Mpf2Ba1 is a 53.2 kDa protein isolated from Pseudomonas monteilii through a multi-step purification process informed by artificial diet bioactivity screening against WCR larvae. The protein is comprised of two domains—an N-terminal MACPF domain and a C-terminal β-prism domain. Pore-forming proteins (PFPs) are a major class of soluble proteins that oligomerize into rings and undergo large irreversible conformational changes to become transmembrane assemblies and breach the membrane of target cells. We have identified and characterized the non-Bt insecticidal protein Mpf2Ba1, providing mechanistic details for how it effectively kills the devastating maize pest WCR by forming pores in midgut membranes targeting a different binding site than the insecticidal proteins currently deployed in commercial transgenic maize hybrids.

A major finding that facilitated Mpf2Ba1 structural characterization is that gut fluid extracted from WCR larvae is necessary and sufficient to induce oligomerization in vitro in the absence of brush-border membrane vesicles (BBMVs) prepared from isolated gut tissue. Upon incubation in gut fluid, an N-terminal cleavage after Lys25, as determined through Edman degradation sequencing, and subsequent oligomerization step are triggered by interaction of monomers with yet unidentified midgut component(s). After gut fluid-induced oligomerization, Mpf2Ba1 monomers formed higher-order complexes that were isolated via size exclusion chromatography and imaged by cryo-EM. The 3D reconstruction of ring-shaped oligomers at 3.1 Å resolution revealed an intermediate state of Mpf2Ba1: a 22-mer pre-pore that is 80 Å in height, 260 Å in diameter, and encircles a 120 Å-wide lumen. By fitting and refining the X-ray structure of Mpf2Ba1 into the pre-pore map, we discovered that we could model the entire protein in the density without breaks, except for the 30 N-terminal residues, five residues more than the 25 identified biochemically. Upon N-terminal removal via gut fluid activation, these contacts are lost and residues on one side of the MACPF domain become fully exposed. The MACPF domain in the Mpf2Ba1 pre-pore remains mostly unchanged, except for loop Val52-Val57 that moves from an external position, in contact with the uncleaved N-terminus, to a buried position in the oligomeric structure, as measured from the accessible surface area per residue. Moreover, it seems that the loop is re-oriented by ~7 Å to bring the highly conserved Ser54 from a solvent-exposed position in the monomer, in contact with His18 of the N-terminus, to a core-buried position towards the MACPF domain in the oligomer. The pre-pore β-prism domain is rotated ~15° clockwise relative to its position in the monomeric structure. This slight rotation disrupts the only interdomain H-bond between MACPF and β-prism, involving the carboxyl oxygen of Glu137 and the hydroxyl group of Tyr460.

>[22x]TVLPGVEAIGLGYNPFISYASVNSGAVQLFDWATAKKREVPFKAGYFVPEIVDVQQNDSATYTNVSGNTISEYQRSLATSVAIEGRYNFFSGSLSTDFDSNSLRNAENEFTRIQQSINLWSLRLPSVKSLRELMLPHMRQQLDELNVNDPKAISRYFDRVGSHFLTGIVMGGRAILASSTNKLRVKRDYSVSVVAKASYEGLTGQLSAEAKAKYGESISSFTQYSNTHQEVRGGDGAKAHGVFSGKKEDFQAWVDSVSASPDFVDFVPTIPMQEIWTLCSSEAQAEAMRKHYDDVWAPAQSEKYRVKANYIDQLVVITGGSSTIEPPVGYSKIEYDLNAGAGGDFIYLCYHEQTWQADRPKDAVTDIRIIFNKEPTPPGYTKLPQDLNKGAGGDDVFLCYKTEAYNTDTAINKVTVIGGNNADINAPYGYLKVPGDLNRGAGGNFIYACTFVGK>MHHHHHHLPNITILATGGTIAGGGDSATKSNYTVGKVGVENLVNAVPQLKDIANVKGEQVVNIGSQDMNDNVWLTLAKKINTDCDKTDGFVITHGTTTMEETAYFLDLTVKCDKPVVMVGAMRPSTSMSADGPFNLYNAVVTAADKASANRGVLVVMNDTVLDGRDVTTTNTTDVATFKSVNYGPLGYIHNGKIDYQRTPARKHTSDTPFDVSKLNELPKVGIVYNYANASDLPAKALVDAGYDGIVSAGVGNGNLYKSVFDTLATAAKTGTAVVRSSRVPTGATTQDAEVDDAKYGFVASGTLNPQKARVLLQLALTQTKDPQQIQQIFNQY[2x]

L-asparaginases catalyze the hydrolysis of L-Asn to L-Asp. The genome of E. coli encodes three L-asparaginases, called type I, II, and isoaspartyl aminopeptidase/L-asparaginase, respectively. The active site pockets of these enzymes are shaped by two protomers, one of which forms most of the active site scaffold, including all catalytic residues; it will be referred to as a “major” protomer, with the second protomer called “minor”. Yet, as we demonstrated here based on the reinterpreted structures of EcAI and the new structures of EcAII, under some conditions a citrate ion can be accommodated into the active site cavity and even displace the canonical substrate or product.

Three structures included in this report, referred to as EcAIID90T/K162T-L-Asn50, EcAIID90T/K162T-L-Asn56, and EcAIID90T/K162T-L-Asn62, were determined for crystals of the EcAIID90T,K162T variant grown in the presence of 10 mM L-Asn at pH 5, 5.6 and 6.2, respectively. All three structures, refined at the resolution of 2.15 Å or higher, are isomorphous and belong to the space group P3121 with two protomers, representing half of the biological assembly, present in the asymmetric unit. We found that the structures are practically invariant within the pH range explored in this study, both in terms of the overall fold as well as details within the active site region. Therefore, we will describe only the structure of EcAIID90T/K162T-L-Asn50. Somewhat unexpectedly, we found that in all three structures one of two independent active sites (in protomer B) was occupied by a citrate anion, despite the fact that L-Asn was present in the crystallization buffer, which is illustrated in Fig. S2c. The position of the citrate in these structures differs significantly from those observed for EcAIIwt-apo7 or for complexes of EcAI. In this case the ligand is stabilized by interactions with the affinity His6-tag, contributed by a symmetry-related protomer, therefore the observed binding mode is an experimental artifact. While the active site appears unoccupied in protomer A, there is a blob of the mFo-DFc electron density adjacent to the side chain of Ser58. Its size, triangular shape and particular location suggest that this peak may represent a carboxylate moiety. Since we cannot unambiguously interpret this electron density, for the purpose of refinement we modeled it as an acetate anion.> KEVWQVILKPKGLGQTKNLIGIYRLCLTSKTISFVKLNSEAAAVVLQLMNIRRCGHSENFFFIEVGRSAVTGPG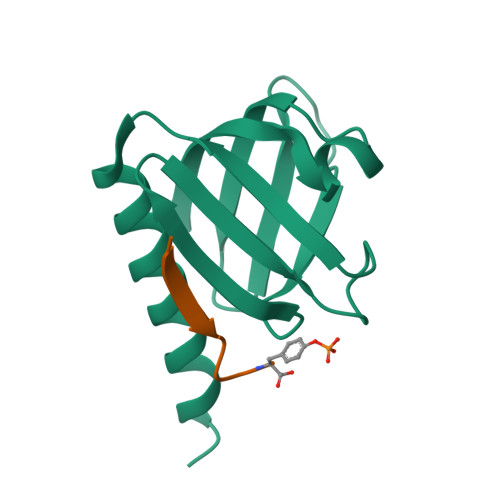EFWMQVDDSVVAQNMHETILEAMRAMSDAFR;> XLYASSNPAY(3-methoxyphenyl)methyl 1~{H}-pyrazole-4-carboxylate 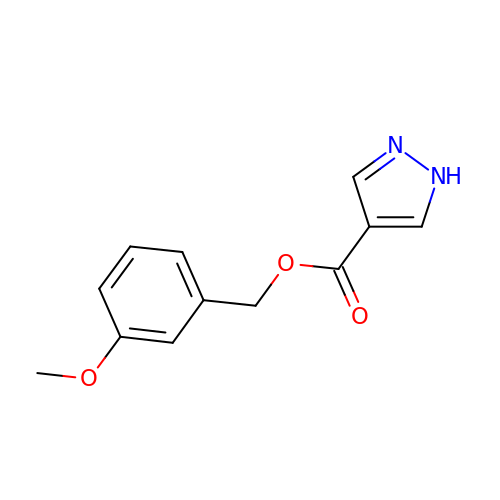| C12 H12 N2 O3 | FPKSPQNXHHFSNA-UHFFFAOYSA-N>VFQKAVDQSIEKKIVLRNGTEAFDSWEKPPLPVYTQFYFFNVTNPEEILRGETPRVEEVGPYTYRELRNKANIQFGDNGTTISAVSNKAYVFERDQSVGDPKIDLIRTLNIPVLTVIEWSQVHFLREIIEAMLKAYQQKLFVTHTVDELLWGYKDEILSLIHVFRPDISPYFGLFYEKNGTNDGDYVFLTGEDSYLNFTKIVEWNGKTSLDWWITDKCNMINGTDGDSFHPLITKDEVLYVFPSDFCRSVYITFSDYESVQGLPAFRYKVPAEILANTSDNAGFCIPEGNCLGSGVLNVSICKNGAPIIMSFPHFYQADERFVSAIEGMHPNQEDHETFVDINPLTGIILKAAKRFQINIYVKKLDDFVETGDIRTMVFPVMYLNESVHIDKETASRLKSMINTHHHHHH[2x]

LIMP-2 is a type III transmembrane glycoprotein encoded by the SCARB2 gene primarily found in lysosomes and late endosomes. LIMP-2 is a receptor for the trafficking of glucocerebrosidase (GCase) from the endoplasmic reticulum to lysosomes, where the acidic environment activates the sphingolipid processing capability of GCase7. LIMP-2 belongs to the class B scavenger receptor family that also includes CD36 and SR-B1. Taken together, these results establish LIMP-2 as a lipid receptor.

We determined a lipid-bound structure of the LIMP-2 luminal domain expressed in HEK cells at 3.0 Å resolution. First, LIMP-2 in our structure forms a symmetric dimer (root-mean-square deviation 0.98 Å for all Cα atoms in the dimer after applying twofold symmetry) via contacts in its two highly distinctive regions of the protein, the α-helical bundle and the region that forms the hydrophobic tunnel. Second, clear electron densities for one phosphatidylcholine (PC) molecule and one CLR molecule were present at the hydrophobic tunnel within each monomer. CLR is completely, and PC partially, buried inside the hydrophobic tunnel. Compared to the reported apo structures, each LIMP-2 subunit has extensive conformational changes that accommodate lipid binding and facilitate protein dimerization. Near the PC head group, D272 and helix α-9 (residues 270–274) are flipped out of the channel to anchor and accommodate the quaternary amine of PC, while K330 and K205 are shifted to contact the phosphodiester of PC. To accommodate CLR, the long loop connecting β9 and β10 (9–10, residues 232–265) flips away and is entirely displaced by the α-helical bundle of the opposite subunit. The displacements/disorder of 9–10, α1, α10, and α11 make the CLR site a much less restricted channel with large openings that connects the distal and the proximal faces of the dimer. In addition to these protein–protein interactions, the acyl chains of the PC molecules bound at both the hydrophobic tunnel and the clefts also contribute extensively to the stabilization of LIMP-2 dimer, explaining the requirement of lipid binding to support dimerization. The expansive mannose-6 glycan, P-Man9GlcNAc2 at N325, makes intermolecular contacts in the dimer.(1S)-1-[1-[3-(4-chlorophenyl)propyl]imidazol-2-yl]ethanol | C14 H17 Cl N2 O | 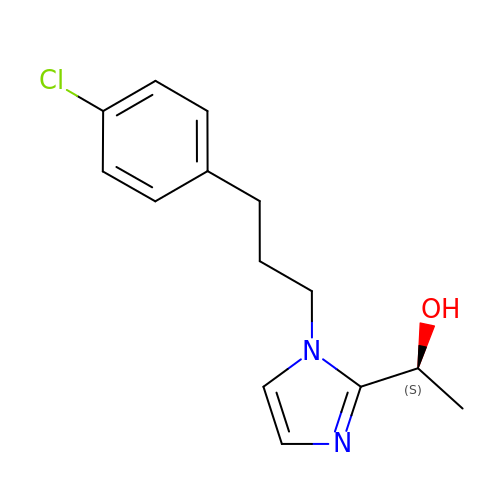GGDYLOWWOJETKU-NSHDSACASA-N>[2x]MSKVPSDIEIAQAAKMKPVMELARGLGIQEDEVELYGKYKAKISLDVYRRLKDKPDGKLILVTAITPTPAGEGKTTTSVGLTDALARLGKRVMVCLREPSLGPSFGIKGGAAGGGYAQVVPMEDINLHFTGDIHAVTYAHNLLAAMVDNHLQQGNVLNIDPRTITWRRVIDLNDRALRNIVIGLGGKANGVPRETGFDISVASEVMACLCLASDLMDLKERFSRIVVGYTYDGKPVTAGDLEAQGSMALLMKDAIKPNLVQTLENTPAFIHGGPFANIAHGCNSIIATKTALKLADYVVTEAGFGADLGA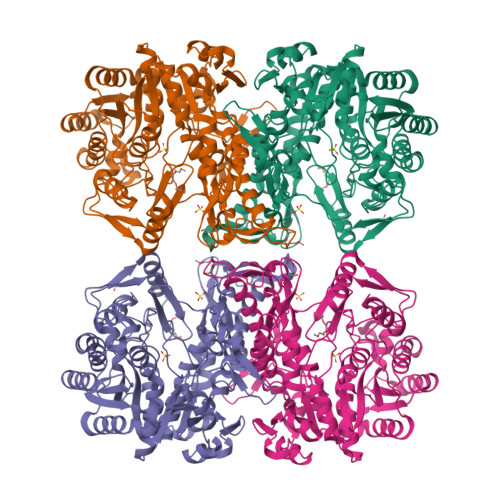EKFYDVKCRYAGFKPDATVIVATVRALKMHGGVPKSDLATENLEALREGFANLEKHIENIGKFGVPAVVAINAFPTDTEAELNLLYELCAKAGAEVALSEVWAKGGEGGLELARKVLQTLESRPSNFHVLYNLDLSIKDKIAKIATEIYGADGVNYTAEADKAIQRYESLGYGNLPVVMAKTQYSFSDDMTKLGRPRNFTITVREVRLSAGAGFIVPITGAIMTMPGLPKRPAACNIDIDADGVITGLF1-(4-HEXYLPHENYL)PROP-2-EN-1-ONE 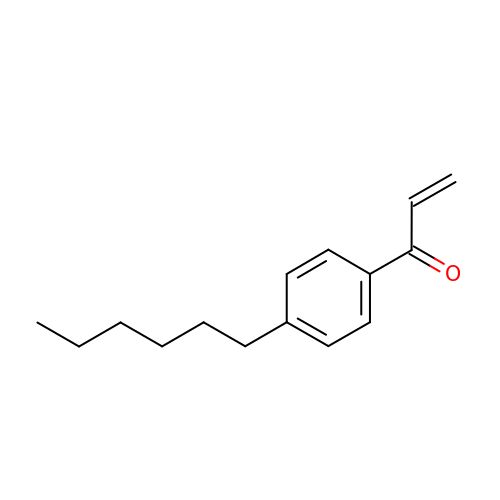| C15 H20 O | IINHTEWASPUCMH-UHFFFAOYSA-N>GSHMEKVPGEME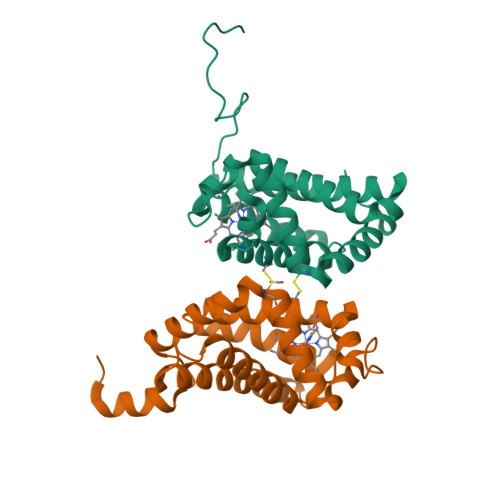IERRERSEELSEAERKAVQAMWARLYANCEDVGVAILVRFFVNFPSAKQYFSQFKHMEDPLEMERSPQLRKHACRVMGALNTVVENLHDPDKVSSVLALVGKAHALKHKVEPVYFKILSGVILEVVAEEFASDFPPETQRAWAKLRGLIYSHVTAAYKEVGWVQQVPNATTPPATLPSSGP[2x]>[4x]MAHHHHHHMT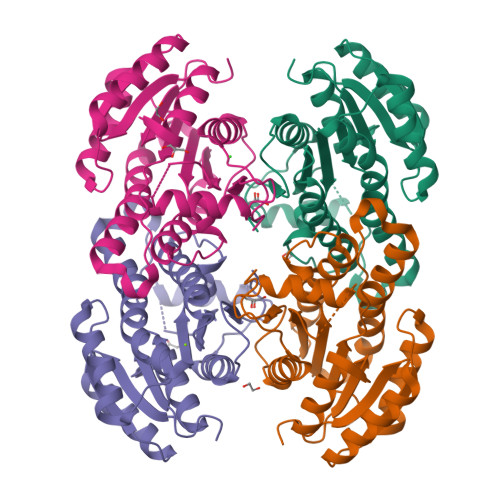APLEGQVAIVTGGARGIGRGIALTLAGAGANILLADLLDDALDATAREVRALGRRAAIAKVDVTQAAQVDAMVAQALADLGGLDILVNCAGVISIHPVAELTERDWDFVMNVNAKGTFLGCRAALAHLKAQGRGRIINVASIAGKEGFPNLAHYSASKFAVVGFTNALAKELARDGVTVNAICPGIVRTYMWDRLSDEWKTDGESVEQSWQRHQLTLIPQGRAQTPEDMGRLALFFATMDNVTGQAVNVDGGFTFH> MSPASPLPVAALSRLRITHRSFLTRSRGRHVCRSAVGVEYRPEQQKKVLDHSYA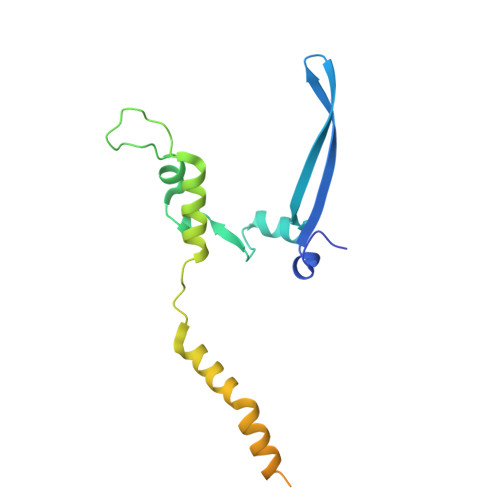RVINAEVVHGDEQKFWGERRTFYTQRNIFFPMWDRCAQALILITREVPRVPQEMAFRLMAVFLKLMLLPRLMMNTELMLPMWIASNAEGAMAAAKDGSKGKEQSSKQQGESKDDAKKEGDNTK> MSTSADYKINQ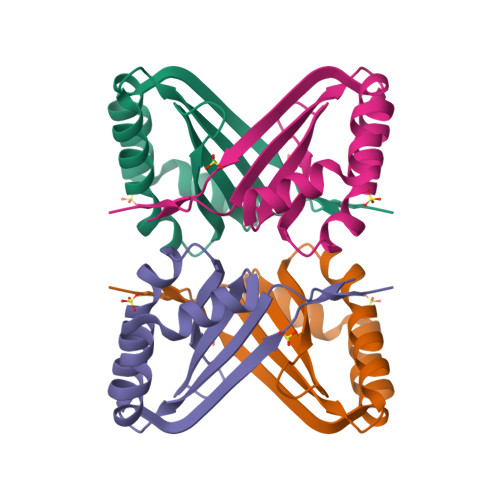QQIVCVASFLSKEGKTEALIAALASLIPDTRREAGCIRYELNVSRDEPRRVTFVEKFVDIAAFDEHCAKDAIQHYFHQVMPELVESFHVETYHQVIA>TEEKTCDLVGEKGKESEKQLALLKRLTPLFQKSFESTVGQSPDMYSYVFRVCREAGQHSSGAGLVQIQKSNGKETVVGRFNETQIFQGSNWIMLIYK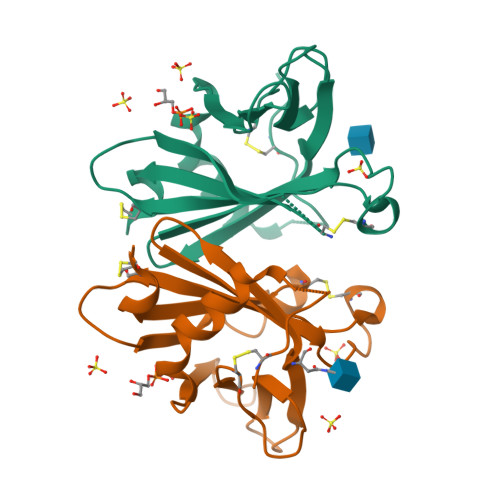GGDEYDNHCGREQRRAVVMISCNRHTLADNFNPVSEERGMVQDCFYLFEMDSSLACS[2x]> MAGQSTHYLAFPRASTITWGDDTRYWSWATVDFSSYAIEEARLLQVSWLDCRWSMD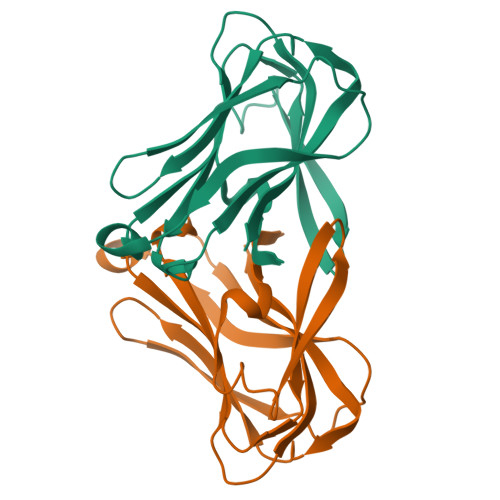ASDFKQDIWYNASVEVMLTSNASGWNVPLHLEIELPDGSKQESQIVLAGRQPNVWFKIPIGKFILRGSLTSGTIRFGFYNHEGNWKRGLNIRTLAIQA>[2x]MAYRDQPLGELALSIPRASALFRKYDMDYAAGGKQTLARAAARKELDVEVIEAELAKLAEQPIEKDWRSAPLAEIIDHIIVRYHDRHREQLPELILQATKVERVH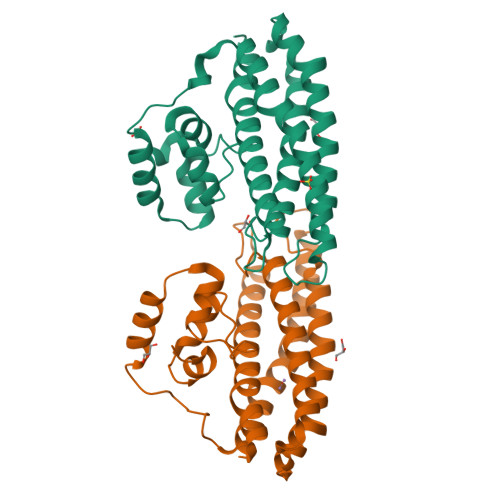ADKPSVPKGLTKYLTMLHEELSSHMMKEEQILFPMIKQGMGSQAMGPISVMESEHDEAGELLEVIKHTTNNVTPPPEACTTWKAMYNGINELIDDLMDHISLENNVLFPRALAGE>MGDSEEPVVTPHAPEFAFDPTDPWTETFQRGLEIAGLGGKRVYEVGIGTGINVAFMLQICEAALVSGSDLDPRLAGLAERNVRDLAPRRADRFHPVEGAVSLIDTPEARAQVGRSDVIVGCLPQVGEPDDVRLRAFRTAQAAALAAGADTRDEDHIAHYYPWAEFDSYPFNSVGLGLNEALLRRTRATAPAADVVLNFGARVGSAVLFELFEANGYVPEKLHSQIVLQHAGTDISFFVALENALAQTGLEREFTCEFYGDPEGATRLSATEAQALVDTDSAAEIYHEVCVIRGRPALSENDPSDS[3x]

MmtN is an S-adenosyl-methionine (SAM)-dependent methyltransferase family enzyme. MmtN catalyzes the S-methylation of Met, in which the methyl group of SAM is transferred to the Met molecule to generate SMM. Recently, diverse marine Actinobacteria, α- and γ-proteobacteria were shown to initiate DMSP synthesis via the methionine (Met) S-methyltransferase enzyme (MmtN), generating S-methyl-Met (SMM). We propose that MmtN uses the proximity and desolvation mechanism for Met S-methylation with two adjacent MmtN monomers comprising the Met binding site.

The best diffraction data was generated using a MmtN K141A/K143A/K146A triple variant from which the crystal structure was solved to 2.5 Å resolution by the single-wavelength anomalous dispersion (SAD) method using a selenomethionine derivative (Se-derivative). Importantly, this MmtN triple variant retained SAM-dependent Met S-methyltransferase activity, exhibiting no substantial difference to the wild-type MmtN enzyme (the specific activities of MmtN and its triple variant were 51.2 ± 1.3 U mmol–1 and 47.3 ± 4.5 U mmol–1, respectively). MmtN crystals belong to a P212121 space group, with three molecules arranged as a trimer in the asymmetric unit. Each MmtN monomer, which is composed of six β-strands and eleven α-helices, consists of a cap domain and a Rossmann-like domain42,43. The MmtN trimer is assembled through interfaces between adjacent monomers, and contains an ion at its center. Ion chromatography measurements implied that the ion in MmtN was a phosphate ion (PO43-), consistent with the result of PO43- detection analysis using the PiColorLock reagent kit (Expedeon, UK). A PO43- is located and likely bound, through electrostatic interactions, to a positively charged ion-binding pocket comprising residues Pro169 and Arg183 in region V of the MmtN monomers. Pro169 and Arg183 are strictly conserved in MmtN, but not in other deposited SAM-dependent methyltransferase structures, suggesting that this ion-binding pocket is unique to MmtN. Therefore, the ion-binding pocket is essential to stabilize the trimer MmtN structure. In the MmtN trimer structure, loop, helixα7, helixα9, and helixα10 of one monomer generate an unclosed hole, and loop of an adjacent MmtN monomer pops out from the Rossmann-like domain to insert into the unclosed hole, resembling a gate latch and bolt pattern.>MGSSHHHHHHSGLVPRGSHMTSKDHVKSQIPRLSAINDLHKIWPTVEEHGAAIIESFLSLDIVRRLNEEVDPFVKIEPIPAAKTKDHPNHVLSTTTRLVNVLAPISKAYREDVLNSKVLHRICSDAFHVYGDYWVLMGAVMELAPSNPAQPLHRDMRFSHPIVEYLKPDAPATSINFLVALSPFTAENGATHVILGSHKWQNLSNVSMDATVRALMNPGDALLITDSTIHCGGAETTGTETRRLLTITMGISQLTPLESNLAVPRPVIESLTPLAQRLLGWASQRSAAPRDIGLLTIRGNSIEKTMNLKAEQPLHDDE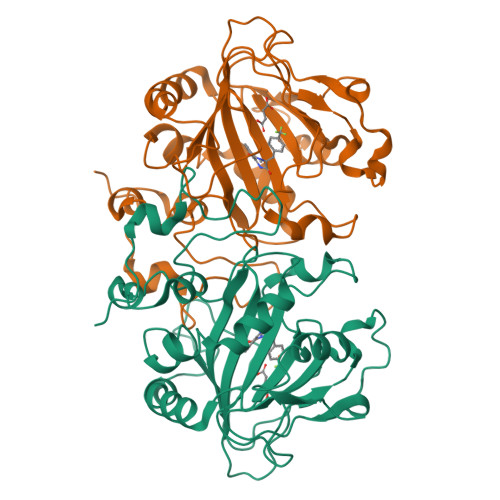AEPLCRETI[2x]> GPLSVAPEMDIMDYCKKEWRGNTQKATCMKMGYEEVSQKFTSIRRVRGDNYCALRATLFQAMSQAVGLPPWLQDPELMLLPEKLISKYNWIKQWK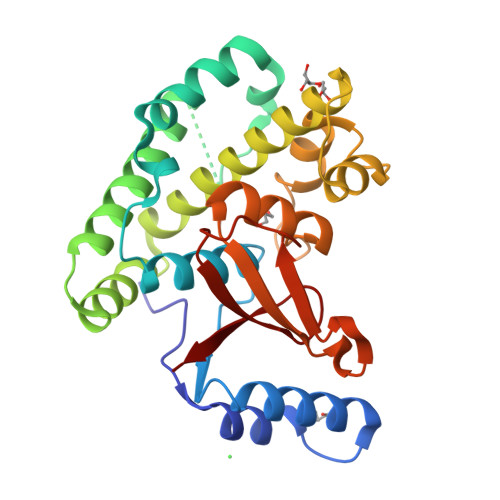LGLKFDGKNEDLVDKIKESLTLLRKKWAGLAEMRTAEARQIACDELFTNEAEEYSLYEAVKFLMLNRAIELYNDKEKGKEVPFFSVLLFARDTSNDPGQLLRNHLNQVRHTGGLEQVEMFLLAYAVRHTIQVYRLSKYNTEEFITVYPTDPPKDWPVVTLIAEDDRHYNIPVR>MKKIAVFTGTRAEYGLLYWLMRDIQQDPELELQILATAMHYSPEHGETWKTIVKDGFEITESVEMLLSSDTSSAVVKSMGVGLLGFADALKRMQPDVLVVLGDRFEALAVTQAALIMHVPVAHLHGGEITEGAYDESIRHAITKMSNIHFAAAEEYKKRIIQLGEQPERVFNVGALGLDHIQRTTFKSISELSELYDFDFSKPYFLITYHPETNLLEENV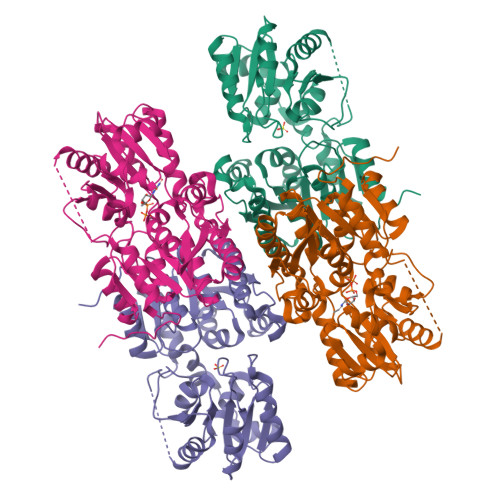APLFDALKQINDVNFIFSYPNADNGNTNIVKAMLDLKAQLPDRVLLVKSFGIQNYLSVLKNALAMVGNSSSGLSEAPALQVPTVNIGDRQKGRLRCESILDVRLDENEIVEALQKAINFPKDQLSQVVPPLGLGNTSQKIIEVIKTTDFKKKAPFYDLLE[4x]> 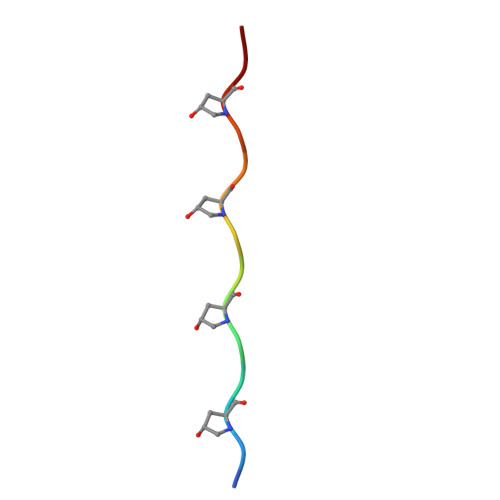GIPGMPGLPGAPGK> SSASFFRPSNPTFGTSISNVQV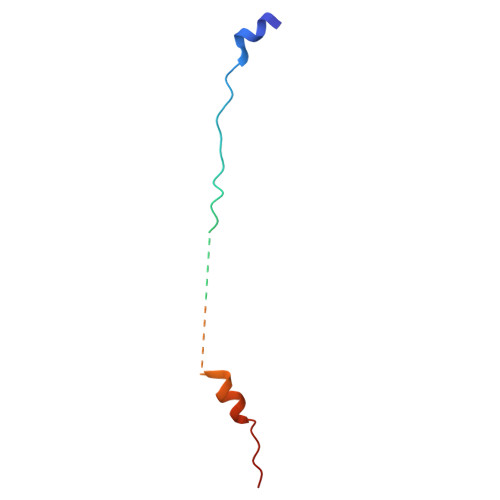NCHPTVAATMAPSRNGPRISSSKALLSSFIARSD> MAGLNEILLPEVHLNSPIVRYKLFYYILHGQLPNDLEPDDLGPLANQNWKAIRAEESQVHARLKQIRVELIARIPSLRWTRSQREIAILIWPRILPILQAYDLRQSMQLPTVWEKLTQSTVNLISDGLERVVLHISNQLTGKPNLFTRSRAGQDTKDYSIPSTRELSQIWFNNEWSGSVKTWLMIKYRMRQLITNQKTGELTDLVTIVDTRSTLCIITPELVALYSSEHKALTYLTFEMVLMVTDMLEGRLNVSSLCTASHYLSPLKKRIEVLLTLVDDLALLMGDKVYGIVSSLESFVYAQLQYGDPVIDIKGTFYGFICNEILDLLTEDNIFTEEEANKVLLDLTSQFDNLSPDLTAELLCIMRLWGHPTLTASQAA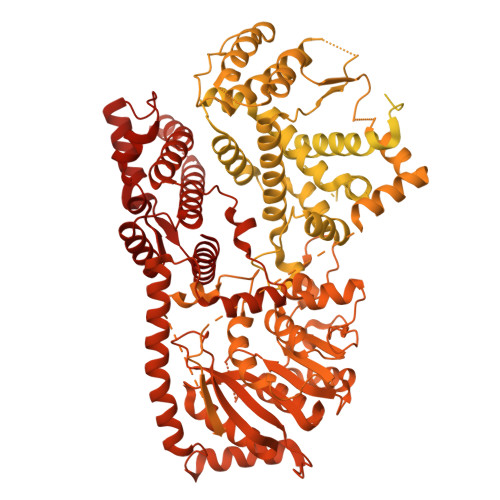SKVRESMCAPKVLDFQTIMKTLAFFHAILINGYRRSHNGIWPPTTLHGNAPKSLIEMRHDNSELKYEYVLKNWKSISMLRIHKCFDASPDEDLSIFMKDKAISCPRQDWMGVFRRSLIKQRYRDANRPLPQPFNRRLLLNFLEDDRFDPIKELEYVTSGEYLRDPEFCASYSLKEKEIKATGRIFAKMTKRMRSCQVIAESLLANHAGKLMRENGVVLDQLKLTKSLLTMNQIGIISEHSRRSTADNMTLAHSGSNKHRINNSQFKKNKDNKHEMPDDGFEIAACFLTTDLTKYCLNWRYQVIIPFARTLNSMYGIPHLFEWIHLRLMRSTLYVGDPFNPPSDPTQLDLDTALNDDIFIVSPRGGIEGLCQKLWTMISISTIILSATEANTRVMSMVQGDNQAIAITTRVVRSLSHSEKKEQAYKASKLFFERLRANNHGIGHHLKEQETILSSDFFIYSKRVFYKGRILTQALKNVSKMCLTADILGDCSQASCSNLATTVMRLTENGVEKDLCYFLNAFMTIRQLCYDLVFPQTKSLSQDITNAYLNHPILISRLCLLPSQLGGLNFLSCSRLFNRNIGDPLVSAIADVKRLIKAGCLDIWVLYNILGRRPGKGKWSTLAADPYTLNIDYLVPSTTFLKKHAQYTLMERSVNPMLRGVFSENAAEEEEELAQYLLDREVVMPRVAHVILAQSSCGRRKQIQGYLDSTRTIIRYSLEVRPLSAKKLNTVIEYNLLYLSYNLEIIEKPNIVQPFLNAINVDTCSIDIARSLRKLSWATLLNGRPIEGLETPDPIELVHGCLIIGSDECEHCSSGDDKFTWFFLPKGIRLDDDPASNPPIRVPYIGSKTDERRVASMAYIKGASVSLKSALRLAGVYIWAFGDTEESWQDAYELASTRVNLTLEQLQSLTPLPTSANLVHRLDDGTTQLKFTPASSYAFSSFVHISNDCQILEIDDQVTDSNLIYQQVMITGLALIETWNNPPINFSVYETTLHLHTGSSCCIRPVESCVVNPPLLPVPLINVPQMNKFVYDPEPLSLLEMEKIEDIAYQTRIGGLDQIPLLEKIPLLAHLTAKQMVNSITGLDEATSIMNDAVVQADYTSNWISECCYTYIDSVFVYSGWALLLELSYQMYYLRIQGIQGILDYVYMTLRRIPGMAITGISSTISHPRILRRCINLDVIAPINSPHIASLDYTKLSIDAVMWGTKQVLTNISQGIDYEIVVPSESQLTLSDRVLNLVARKLSLLAIIWANYNYPPKVKGMSPEDKCQALTTHLLQTVEYVEYIQIEKTNIRRMIIEPKLTAYPSNLFYLSRKLLNAIRDSEEGQFLIASYYNSFGYLEPILMESKIFNLSSSESASLTEFDFILNLELSDASLEKYSLPSLLMTAENMDNPFPQPPLHHVLRPLGLSSTSWYKTISVLNYISHMKISDGAHLYLAEGSGASMSLIETFLPGETIWYNSLFNSGENPPQRNFAPLPTQFIESVPYRLIQAGIAAGNGIVQSFYPLWNGNSDITDLSTKTSVEYIIHKVGADTCALVHVDLEGVPGSMNSMLERAQVHALLITVTVLKPGGLLILKASWEPFNRFSFLLTVLWQFFSTIRILRSSYSDPNNHEVYIIATLAVDPTTSSFTTALNRARTLNEQGFSLIPPELVSEYWRKRVEQGQIIQDCIDKVISECVRDQYLADNNIILQAGGTPSTRKWLDLPDYSSFNELQSEMARLITIHLKEVIEILKGQASDHDTLLFTSYNVGPLGKINTILRLIVERILMYTVRNWCILPTQTRLTLRQSIELGEFRLRDVITPMEILKLSPNRKYLKSALNQSTFNHLMGETSDILLNRAYQKRIWKAIGCVIYCFGLLTPDVEGSERIDVDNDIPDYDIHGDII> DPSDRLVPELDTIVPLESTKAYNMVDIIHSVVDEREFFEIMPNYAKNIIVGFARMNGRTVGIVGNQPKVASGCLDINSSVKGARFVRFCDAFNIPLITFVDVPGFLPGTAQEYGGIIRHGAKLLYAFAEATVPKVTVITRKAYGGAYDVMSSKHLCGDTNYAWPTAEIAVMGAKGAVEIIFKGHENVEAAQ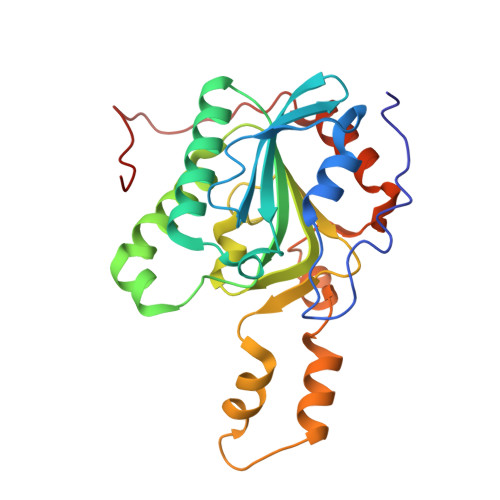AEYIEKFANPFPAAVRGFVDDIIQPSSTRARICCDLDVLASKKVQRPWRKHANIPL1-[4-(4-ethylpiperazin-1-yl)-3-fluorophenyl]butan-1-one | C16 H23 F N2 O | 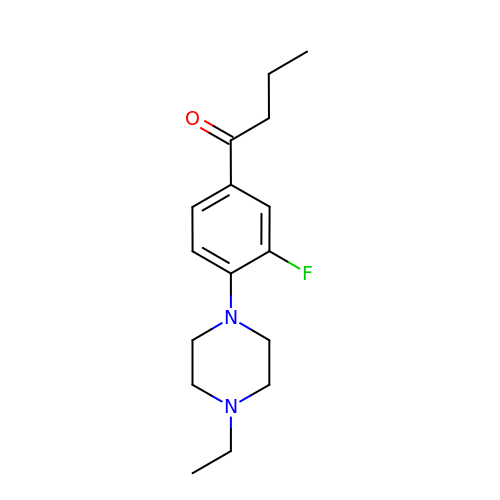IYDDEPAMENQFDL-UHFFFAOYSA-N> ATQQEICKNMWDPFQSMRAVTGLMELTSGQCTQLSKDAAAILAGVKESHDSISVDKNYKVLNDEVAYHAANIDAAAKANDLEEVQVQFRRMTIACRNCHKIYKTEQRLVP;> LNEHTAGDTTK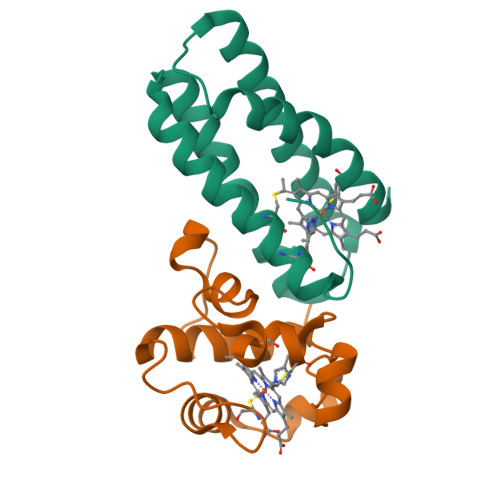SPYTIYAGLGFAVQESCYYCHGNGGKGTTEGLIFGVPDFTSTEFQSSMTDKQIIDHINKGKGKCPSYQGKMSPEMIEKMAGVVRNFAVK> SVKVGGEAGPSVTLPCHYSGAVTSMC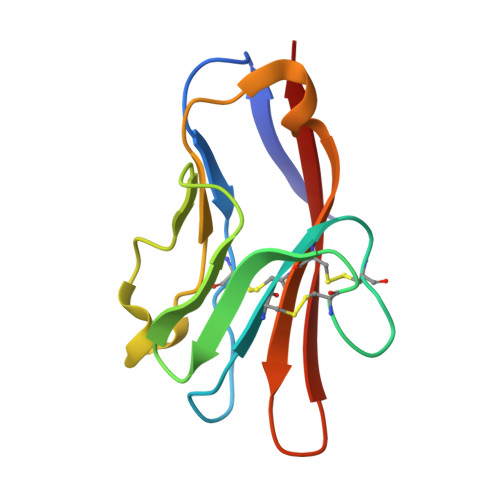WNRGSCSLFTCQNGIVWTNGTHVTYRKDTRYKLLGDLSRRDVSLTIENTAVSDSGVYCCRVEHRGWFNDMKITVSLE> ADAPAGTDPRAK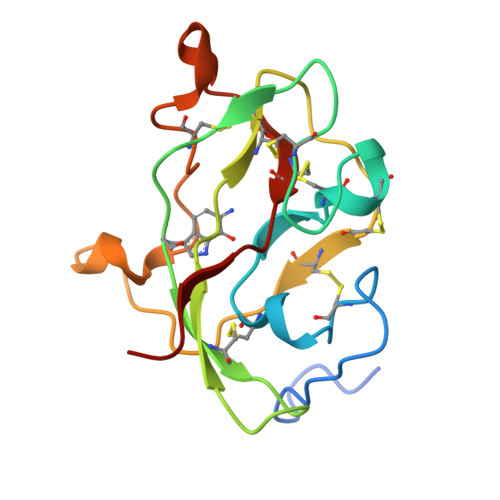WVPQDNDIQACDYWRHCSIDGNICDCSGGSLTNCPPGTKLATASWVASCYNPTDGQSYLIAYRDCCGYNVSGRCPCLNTEGELPVYRPEFANDIIWCFGAEDDAMTYHCTISPIVGKAS(2S)-2-HYDROXYOCTANOIC 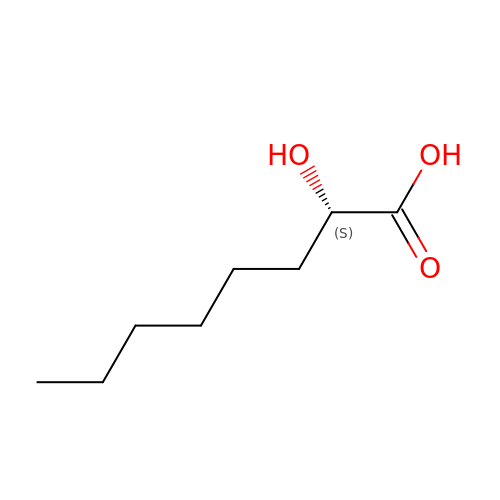ACID | C8 H16 O3 | JKRDADVRIYVCCY-ZETCQYMHSA-N> GPGSMLI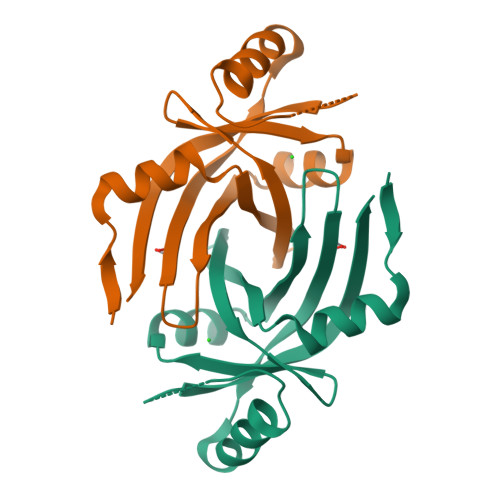TEMSDYDIREMIQHKHVGRLGYVVDDRPIIVPMTFRFSGGSFYSFTTDGQKTNAMRKNDAICILFDQIESQTKWRTVLVQGRYREIAREDEEEAIVRIMANEPTWWEPAYTKTITKEGTARALKPVFFRVDIEKLSGHQAE>TGYLTQEEIALLLAALDGDNKKIAILCLSTGARWGEAARLKAENIIHNRVTFVKT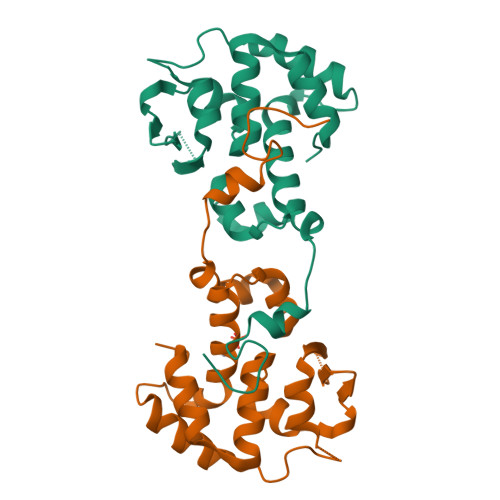KTNKPRTVPISEAVAKMIADNKRGFLFPDADYPRFRRTMKAIKPDLPMGQATHALRHSFATHFMINGGSIITLQRILGHTRIEQTMVYAHFAPEYLQDAISLNPLRGGTEAESVHTVSTVE[4x]HSP100 unfoldases, a subclass of the AAA chaperones found in yeast and bacteria as well as in the mitochondria and chloroplasts of higher eukaryotes, employ a powerful mechanism to recover functional proteins from aggregates. Upon forming a hexameric ring, they unravel polypeptides by threading them through a narrow central pore. To avoid damage to native proteins, the high unfolding potential of Hsp104 and related disaggregases needs to be carefully regulated. This control is mediated by an inserted coiled-coil domain (M-domain, MD), which assembles a molecular belt encircling the hexameric particle and keeping the enzyme in its latent state. The Hsp104 disaggregase is composed of tandemly linked structural modules that build up the N-terminal domain (NTD), the two ATPase engines (AAA1, AAA2), and the regulatory MD extension.

Here, we present the crystal structure of Hsp104 from Chaetomium thermophilum that – although forming a helical filament – reveals important mechanistic features. The crystal structure of the double Walker-B mutant in complex with ADP was determined at 3.7 Å resolution. In the crystal, CtHsp104 subunits are arranged in a helical 61 filament rather than forming a defined hexameric particle as observed in the recent cryo-electron microscopy structure of ScHsp104 or the crystal structure of a related HSP100 unfoldase, ClpC. Although the obtained crystals are formed by the full-length protein (data not shown), the NTD was not defined by electron density, likely due to high flexibility. The active sites, located at the AAA subdomain interface, are defined by co-crystallized ADP molecules, which were clearly visible in the electron density map. Importantly, however, the crystallized filament seems to reflect mechanistic properties of the HSP100 hexamer, as the architecture of the basic building blocks of AAA unfoldases, the so-called rigid bodies, is comparable to that in both ClpC and ScHsp104 hexameric structures. The present crystal structure provides a detailed picture of the resting state of Hsp104, shedding light on the regulatory role of the MD. In parallel, the MD binds to the neighboring ATPase module by docking the tip of motif-2, particularly Arg509, into a two-helix cleft on the edge of the AAA1 large subdomain. Strikingly, in the crystal structure of Hsp104, the PS1-hairpin protrudes from the AAA2 into the AAA1* ring, where it is accommodated in a deep pocket close to the ATP binding site of a neighboring subunit. At the tip of the PS1-haripin, the side chains of Gln732 and Arg734 form specific interactions with Asp406* and Asp410* located on the sensor-2 helix.

>MNSKMEFTDRAKKALEDAMALAEQYQHLQLQPVHLAVALLDPTPDPSKDQSIAPGTTSTLFRQVVERAHGDAQAFDRALKKKLVRLPSQDPPPDQVSMSAGCSNVLRKANELQKVQKDSYIAVDHLIAALAEDHAIQEALKEANIPKPKLIQDAIQAIRGNKRVDSRNADTEQENENLSKFCIDMTAMAREGKIDPVIGREEEIRRVIRILSRRTKNNPVLIGEPGVGKTTIVEGLAQRIVNADVPDNLAACKLLSLDVGALVAGSKYRGEFEERMKGVLKEIQESKETIILFVDAIHLLMGAGSSGEGGMDAANLLKPMLARGQLHCIGATTLAEYRKYIEKDAAFERRFQQVLVKEPSISETISILRGLKEKYEVHHGVNIADAAIVAAANLAARYLTSRRLPDSAVDLIDEAAAAVRVARESQPEIIDSLERRLRQLKIEIHALSREKDEASKARLAQAKQDAQNVEEELRPLREKYERERQRGKAIQEAKMKLEALRVKAEDASRMGDHSRAADLQYYAIPEQEAIIKRLEAEKAAADAALNANGADVGGSMITDVVGPDQINEIVARWTGIPVTRLKTSEKEKLLHMEQALSKIVVGQKEAVQSVSNAIRLQRSGLSNPNQPPSFLFCGPSGTGKTLLTKALAEFLFDDPKSMIRFDMSEYQERHSLSRMIGAPPGYVGHDAGGQLTEALRRRPFSILLFDAVEKAAKEVLTVLLQLMDDGRITDGQGRVVDAKNCIVVMTSNLGAEYLSRANNGKDGKIDPTTRELVMNTLRNYFLPEFLNRISSVVIFNRLTRREIRKIVDLRIAEIQKRLTDNDRNVIIKVSEEAKDKLGAQGYSPVYGARPLQRLLEKEVLNRLAILILRGQIREGEVAHVELVDGKVQVLPNHPDSEPEDVDVDMDSDDAVDEVAPDSMDEDIYND[3x]> LENGLARTPP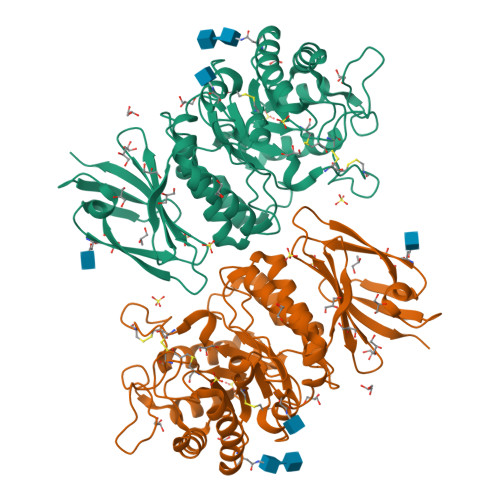MGWLAWERFRCNVNCREDPRQCISEMLFMEMADRIAEDGWRELGYKYINIDDCWAAKQRDAEGRLVPDPERFPRGIKALADYVHARGLKLGIYGDLGRLTCGGYPGTTLDRVEQDAQTFAEWGVDMLKLDGCYSSGKEQAQGYPQMARALNATGRPIVYSCSWPAYQGGLPPKVNYTLLGEICNLWRNYDDIQDSWDSVLSIVDWFFTNQDVLQPFAGPGHWNDPDMLIIGNFGLSYEQSRSQMALWTIMAAPLLMSTDLRTISPSAKKILQNRLMIQINQDPLGIQGRRIIKEGSHIEVFLRPLSQAASALVFFSRRTDMPFRYTTSLAKLGFPMGAAYEVQDVYSGKIISGLKTGDNFTVIINPSGVVMWYLCPKALLIQQQAPGGPSRLPLL(3R)-4-{[(3,4-dihydroxyphenyl)acetyl]oxy}-N-(2-formylindolizin-3-yl)-3-sulfino-D-valine 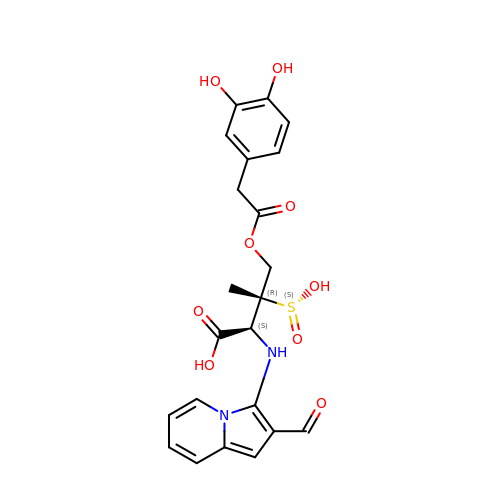| C22 H22 N2 O9 S | DEOZLEGRVHDNKC-UGKGYDQZSA-N> MRVLVTGGSGYIGSHTCVQLLQNGHDVIILDNLCNSKRSVLPVIERLGGKHPTFVEGDIRNEALMTEILHDHAIDTVIHFAGLKAVGESVQKPLEYYDNNVNGTLRLISAMRAANVKNFIFSSSATVYGDNPKIPYVESFPTGTPQSPYGKSKLMVEQILTDLQKAQPDWSIALLRYFNPVGAHPSGDMGEDPQGIPNNLMPYIAQVAVGRRDSLAIFGNDYPTEDGTGVRDYIHVMDLADGHVVAMEKLANKPGVHIYNLGAGVGNSVLDVVNAFSKACGKPVNYHFAPRREGDLPACWADASKADR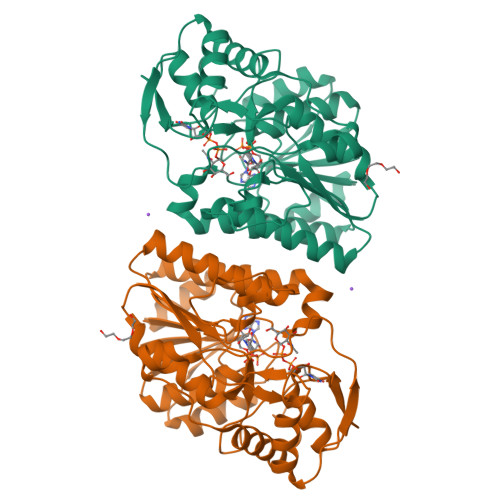ELNWRVTRTLDEMAQDTWHWQSRHPQGYPD(2E)-3-{5-[(2,4-diamino-6-ethylpyrimidin-5-yl)methyl]-2,3-dimethoxyphenyl}-1-[(1S)-1-(2-methylprop-1-en-1-yl)phthalazin-2(1H)-yl]prop-2-en-1-one 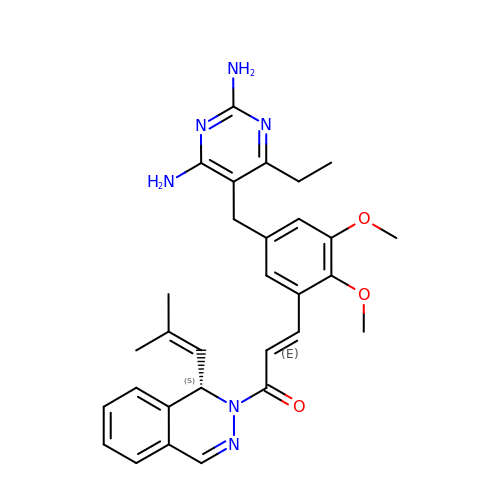| C30 H34 N6 O3 | CWIYQEZJRSEBAE-CJZRDCOESA-N>GSKPHQWQADEEAVRSATCSFSVKYLGCVEVFESRGMQVCEEALKVLRQSRRRPVRGLLHVSGDGLRVVDDETKGLIVDQTIEKVSFCAPDRNHERGFSYICRDGTTRRWMCHGFLACKDSGERLSHAVGCAFAVCLERKQ[2x];>[2x]QQKLPTNPFEVLRQPPKKKKREHACFENPGLNLE

As the first identified cell fate determinant, Numb transiently forms a basal crescent during mitosis, preferentially segregates to the basal GMC daughter, and then promotes its differentiation to neurons/glia by antagonizing Notch signaling. During NB division, Pon together with Numb is basally localized and is segregated into the basal daughter cell. We found that Numb PTB specifically recognizes the AB motif repeats of its adaptor Pon in a previously unrecognized manner. The multivalent interaction between Numb and Pon can lead to LLPS of the complex, forming condensed, autonomously assembled membrane-lacking compartments both in vitro and in living cells.

Several repeating motifs have been found in Pon1-228: type A “FxNxx[F/L]” motif and type B “NP[F/Y]E[V/I]xR” motif. Proper combination of both motifs dramatically increased the interaction with Numb PTB, whereas the isolated one barely bound to it. For example, Pon fragments containing either B1A2, A2B2, or A3B3 showed significantly enhanced binding avidity to PTB compared with the isolated A or B motifs. To elucidate how combination of A and B motifs can strengthen Pon’s binding to Numb PTB, we solved the crystal structures of Numb PTB in complex with Pon A2B2 or Pon B1A2 peptides. The complex structures revealed that either Pon A2B2 or Pon B1A2 binding led PTB to form a symmetric dimer-of-dimers in either a “head-to-head” or “tail-to-tail” organization. Pon binding could also induce Numb dimerization in solution. Despite of the distinct domain arrangement in the two complexes, the A or B motifs from B1A2 and A2B2 occupied the identical sites on PTB. For example, the bulky aromatic ring of Tyr154B2 (same as Phe120B1) inserts into a hydrophobic pocket formed by the side chains of Tyr87, Val117, and Ile139 from PTB. The side chain of Arg158B2 (same as Arg124B1) forms hydrogen bonds with the backbone carbonyl oxygen of Glu92PTB. By analyzing all the PTB or PTB/ligand structures deposited in the Protein Data Bank, we further found that the newly identified B motif-binding hydrophobic pocket on the Drosophila Numb PTB appears to be present in most of other PTB domains.>VETISFSFSEFEPGNNDLTLQGAAIITQSGVLQLTKINQNGMPAWDSTGRTLYTKPVHIWDMTTGTVASFETRFSFSIEQPYTRPLPADGLVFFMGPTKSKPAQGYGYLGVFNNSKQDNSYQTLAVE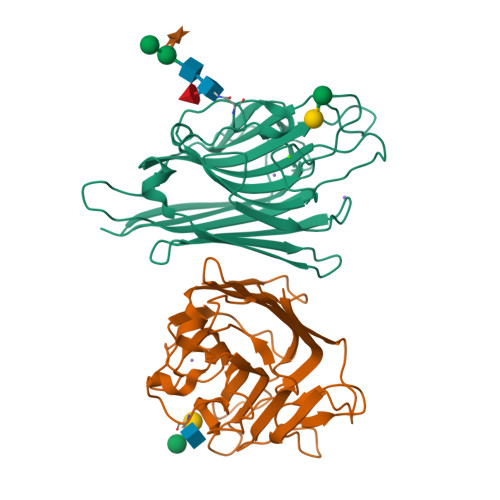FDTFSNPWDPPQVPHIGIDVNSIRSIKTQPFQLDNGQVANVVIKYDASSKILLAVLVYPSSGAIYTIAEIVDVKQVLPEWVDVGLSGATGAQRDAAETHDVYSWSFHASLPE[2x]DIPHOSPHOMETHYLPHOSPHONIC ACID ADENOSYL 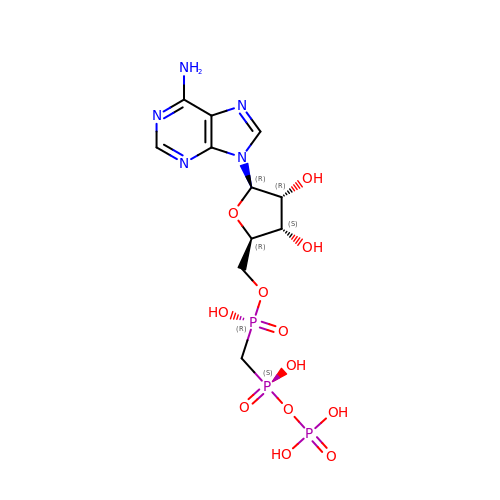ESTER | C11 H18 N5 O12 P3 | CAWZRIXWFRFUQB-IOSLPCCCSA-N>MGRDPNSTNDTTTQNVVLTKYGFDKDVTAIDRATDQIWTGDGAKPLQGVDFTIYNVTANYWASPKDYKGSFDSAPVAATGTTNDKGQLTQALPIQSKDASGKTRAAVYLFHETNPRAGYNTSADFWLTLPAKAAADGNVYVYPKNVQKTTYERTFVKKDAETKEVLEGAGFKISNSDGKFLKLTDKDGQSVSIGEGFIDVLANNYRLTWVAESDATVFTSDKSGKFGLNGFADNTTTYTAVET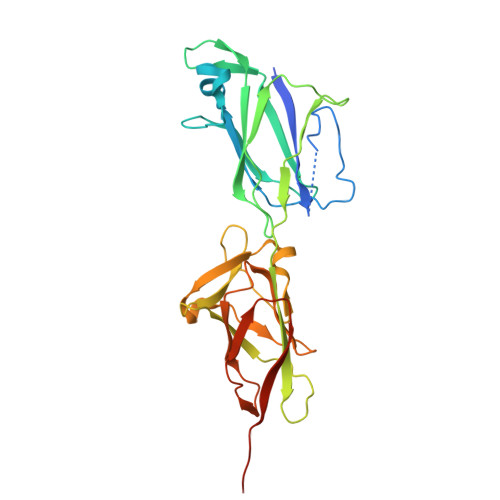NVPDGYDAAANTDFKADNSSSDILNAPSGILPLEHHHHHH[6x]>GICKSSDCIKSAARLIQNMDATTEPCTDFFKYACGGWLKRNVIPETSSRYGNFDILRDELEVVLKDVLQEPKTEDIVAVQKAKALYRSCINESAIDSRGGEPLLKLLPDIYGWPVATENWEQKYGASWTAEKAIAQLNSKYGKKVLINLFVGTDDKNSVNHVIHIDQPRLGLPSRDYYECTGIYKEACTAYVDFMISVARLIRQEERLPIDENQLALEMNKVMELEKEIANATAKPEDRNDPMLLYNKMTLAQIQNNFSLEINGKPFSWLNFTNEIMSTVNISITNEEDVVVYAPEYLTKLKPILTKYSARDLQNLMSWRFIMDLVSSLSRTYKESRNAFRKALYGTTSETATWRRCANYVNGNMENAVGRLYVEAAFAGESKHVVEDLIAQIREVFIQTLDDLTWMDAETKKRAEEKALAIKERIGYPDDIVSNDNKLNNEYLELNYKEDEYFENIIQNLKFSQSKQLKKLREKVDKDEWISGAAVVNAFYSSGRNQIVFPAGILQPPFFSAQQSNSLNYGGIGMVIGHDITHGFDDNGRNFNKDGDLVDWWTQQSASNFKEQSQCMVYQYGNFSWDLAGGQHLNGINTLGENIA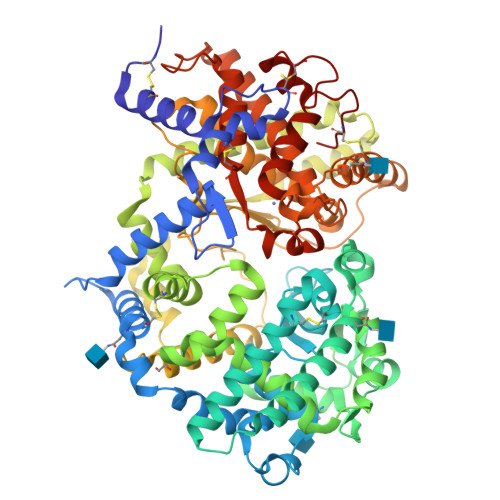DNGGLGQAYRAYQNYIKKNGEEKLLPGLDLNHKQLFFLNFAQVWCGTYRPEYAVNSIKTDVHSPGNFRIIGTLQNSAEFSEAFHCRKNSYMNPEKKCRVW[2x]> MPLKRSLKESIERLSSFQSKYNIFTSINPSPYSITNKKGTKETLTGCVASIKDNIVTKDFPTTCASHILENFKSPFDATVVKLLKQAGVHILGKTNLDEFGMGSGGVHSIRGPVINPLYPHEDKKIMGGSSSGAAASVACDLVDFALGTDTGGSVRLPACYGSVLGFKPSYGRLSRFGVIAYSQSLDTVGILSKKINVLRKVFHTLDKYDMKDPTSLSVELRELIEGNKKVRRPLKVGIVKEFSHESMPIGFHRLYLSLLEKLINLGLEIYPVSIPSVKNCLPIYYTLSPAEAASNLSRYDGIRYGYRDSELDIKDGILFAPTRSKFGTEVKNRIILGNYNLCSDAFKNNFIKAEKLRVNLIDEFDGIFRFPNVLTNSKGNPDGLDLLIVPTSSKLPGSIRDFEEEEAKSPANSYINDVFTVPMSLAGLPSLSMPLKEKTPIGLQVVGQYGDDSTVLDFVESIS;> IHSHGAPFRPEYALKCGLEIHTQLNTKNKLFSQSTNSATSLVDAPNHHTSYYDIALPGTQPVLNLEAILFAMKLSLALGSQVNSISQFDRKHYFYGDQPQGYQLTQHYRPFARGGKINLSKELDDIDESAKEIGILQLQIEQDTGKSHYTETDKDVITLVDLNRSNVPLIELVTKPDFSDIKQVRAFIKKYQNLVRHLHISSGDLETGAMRVDVNLSINEYARVELKNLPNTSSIINAIKYEYQRQVELISVGDTSSLMEPETRGWTGSSTVKLRSKETTIDYRYMPDPELPYINLAPDVISGVRGLMPQLPDDLESSGENLYFQ;> FVSTGGAKIGKKFENMNQIRDYLSRPVWSVHEYLGINTKEEKLEPPSAEAVKKLLRLSGLPLEGADIKEIQMRLAKQLSFINKLHNIPVEGEKHTKEYDARLVQRNTKQLNYTKLLEGISHQKQDAELGEVSGSWKATGLAAESKNAYFVVKEGLLKNRK

Our recent study revealed that yeast Gln-mtRNAGln is synthesized by a transamidation pathway involving a novel heterotrimeric AdT named GatFAB. GatA hydrolyzes Gln into Glu and an ammonia molecule, which travels to GatB through an intramolecular ammonia tunnel. The third subunit, GatF, is a new type of AdT subunit found only in fungal genomes. While the GatC-like portion encircles the GatA–GatB contact area, the NTD forms extended interactions with the GatA core domain.

To facilitate crystallization, the putative N-terminal mitochondrial targeting sequences of GatB (residues 1–15) and GatF (residues 1–23) were eliminated. Furthermore, we truncated the C-terminal helical and YqeY domains (residues 330–474 and 475–541, respectively), which were reported to be highly flexible. The crystal structure of the heterotrimeric GatFAB AdT from S. cerevisiae was determined by the multiple wavelength anomalous diffraction method. The final models of the free and glutamine-bound forms were refined at 2.0 Å resolutions to free R-factors of 22.2 and 21.9%, respectively. Intriguingly, the side chain of H54 is disordered in the apo form structure, while all of the other hydrophilic and hydrophobic interactions between GatF and GatA are preserved in both the Gln-bound and free forms. Based on the superposition of our structure with that of the bacterial GatCAB, the yeast GatF can be divided into two halves, the C-terminal GatC-like portion and the N-terminal appended domain (NTD). The linker loop connecting the NTD and the C-terminal GatC-like structure is completely disordered, reflecting the flexibility of the NTD. In contrast, we were not able to identify any substrate in the AdT site of GatB, whereas S. aureus and A. aeolius GatB structures co-crystallized with ATP or its analogues. Inside this tunnel are several electron densities corresponding to water molecules, or possibly ammonia.> STGSATTTPIDSLDDAYITPVQIGTPAQTLNLDFDTGSSDLWVFSSETTASEVDGQTIYTPSKSTTAKLLSGATWSISYGDGSSSSGDVYTDTVSVGGLTVTGQAVESAKKVSSSFTEDSTIDGLLGLAFSTLNTVSPTQQKTFFDNAKA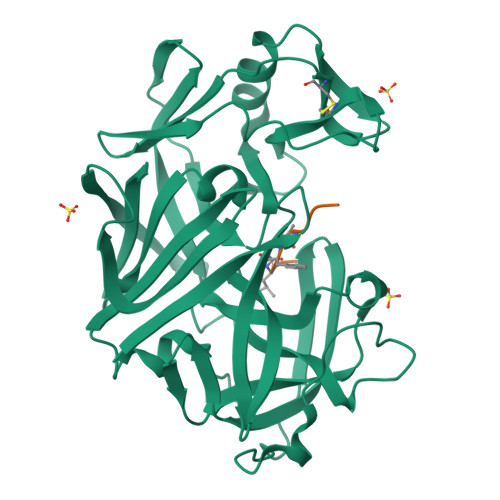SLDSPVFTADLGYHAPGTYNFGFIDTTAYTGSITYTAVSTKQGFWEWTSTGYAVGSGTFKSTSIDGIADTGTTLLYLPATVVSAYWAQVSGAKSSSSVGGYVFPCSATLPSFTFGVGSARIVIPGDYIDFGPISTGSSSCFGGIQSSAGIGINIFGDVALKAAFVVFNGATTPTLGFASK;> TFQAFLRE>[2x]MVTSPALRDVHVPHAYPEQQVDLGEITMNYAEAGDPDR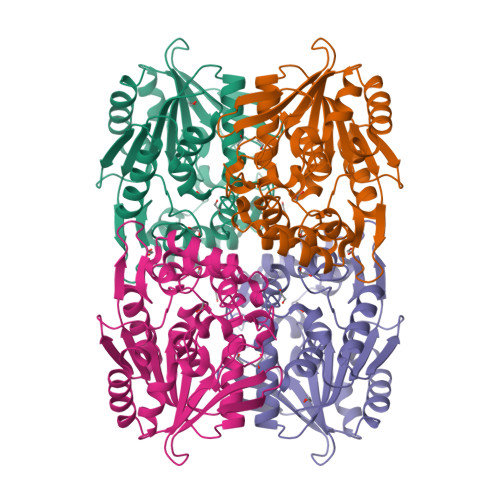PAVLLIPEQTGSWWSYEEAMGLLSEHFHVYAVDLRGQGRSSWTPKRYSLDNFGNDLVRFIALVVKRPVVVAGNSSGGVLAAWLSAYSMPGQLRGVLCEDPPFFASELVPAHGHSVRQGAGPVFELFRTYLGDQWSVGDWEGFCRAAGASASPMARSFVADGIPQHLQEYDPEWARVFYEGTVGLSCPHERMLGQVKTPVLLTHHMRGIDPETGNLLGALSDEQALRARRLMDSAGVTVDYESVPDASHMMHQSAPARYVEIFTRWAAALAPHHHHHH>[4x]SYQSLKNKVVIVTGAGSGIGRAIAKKFALNDSIVVAVELLEDRLNQIVQELRGMGKEVLGVKADVSKKKDVEEFVRRTFETYSRIDVLCNNA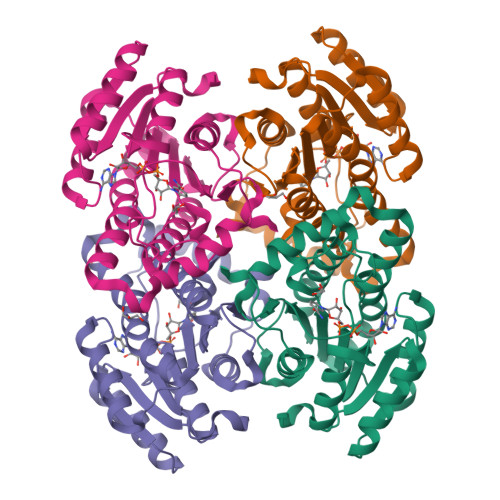GIMDGVTPVAEVSDELWERVLAVNLYSAFYSSRAVIPIMLKQGKGVIVNTASIAGIRGGFAGAPYTVAKHGLIGLTRSIAAHYGDQGIRAVAVLPGTVKTNIGLGSSKPSELGMRTLTKLMSLSSRLAEPEDIANVIVFLASDEASFVNGDAVVVDGGLTVL>[2x]MTAPRPSKIRLGNHLLHPETQMLNYGYDSELSEGAVKPPVFLTSTFVFKTAEDGRDFFDFVSGRKEPPAGVGAGLVYSRFNHPNSEIVEDRLAVYEGAESAALFSSGMSAIATTLFAFVRPGDVILHSQPLYGGTETLLAKTFFNFGVEAVAFADGVHEATIEKAAEEALAKGRVSVILIETPANPTNSIVDVAAVRRVAEKIEARQGSRPVIACDNTLLGPVFQ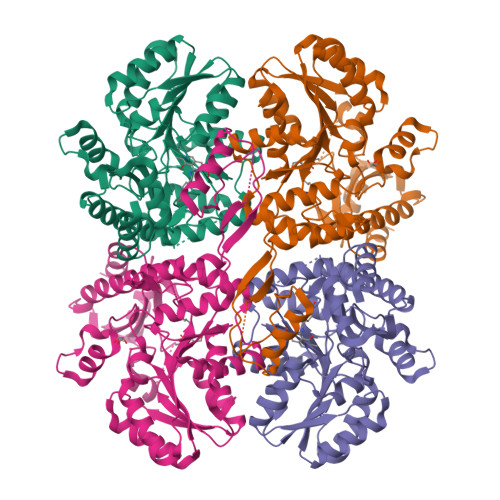KPLDHGADLSVYSLTKYVGGHSDLIAGAVLGAKSVVRQVKALRGAIGTQLDPHSCWMLGRSLETLGLRMERADSNARAIAEFLRNHPKVEKLHYLPFADERSDIAALFKRQCTGAGSTFSFDIKGGQAAAFRFLNALQILKLAVSLGGTESLASHPAAMTHSGVPVDVRERIGVLESTIRLSIGIEHPDDLIADLAQALDAA> ACCGUCAGAG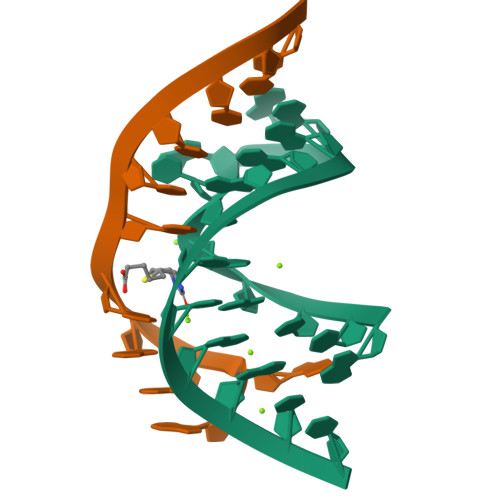GACACGGUU;> AAAAAGUCCUC> MGQSKKLNKQPSSLSPLVQLAGIRKCFDGKEVIPQLDLTINNGEFLTLLGPSGCGKTTVLRLIAGLETVDSGRIMLDNEDITHVPAENRYVNTVFQSYALFPHMTVFENVAFGLRMQKTPAAEITPRVMEALRMVQLETFAQRKPHQLSGGQQQRVAIARAVVNKP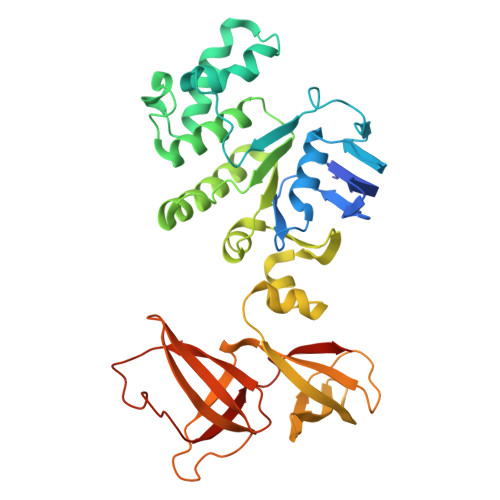RLLLLDQSLSALDYKLRKQMQNELKALQRKLGITFVFVTHDQEEALTMSDRIVVMRDGRIEQDGTPREIYEEPKNLFVAGFIGEINMFNATVIERLDEQRVRANVEGRECNIYVNFAVEPGQKLHVLLRPEDLRVEEINDDNHAEGLIGYVRERNYKGMTLESVVELENGKMVMVSEFFNEDDPDFDHSLDQKMAINWVESWEVVLADEEHK> MAMLYLIFYDITDDNLRNRVAEFLKKKGLDRIQYSVFMGDLNSSRLKDVEAGLKIIGNRKKLQE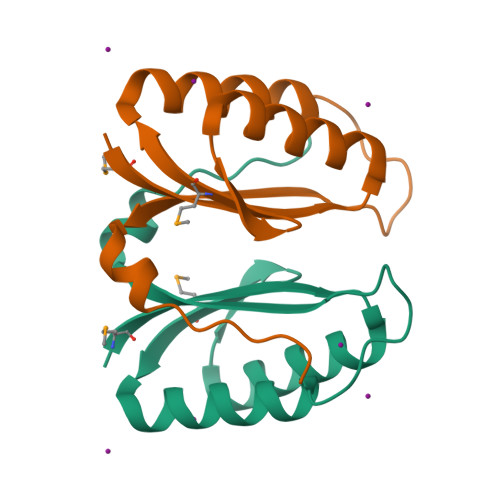DERFFILIVPITENQFRERIVIGYSGSEREEKSNVVW>GFGCNGPWSEDDMKCHNHCKSIK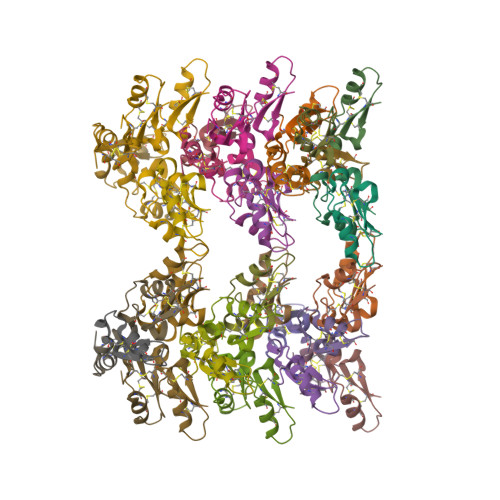GYKGGYCAKGGFLCKCY[42x]>[2x]MFQQLSARLQEAIGRLRGRGRITEEDLKATLREIRRALMDADVNLEVARDFVERVREEALGKQVLESLTPAEVILATVYEALKEALGGEARLPVLKDRNLWFLVGLQGSGKTTTAAKLALYYKGKGRRPLLVAADTQRPAAREQLRLLGEKVGVPVLEVMDGESPESIRRRVEEKARLEARDLILVDTAGRLQIDEPLMGELARLKEVLGPDEVLLVLDAMTGQEALSVARAFDEKVGVTGLVLTKLDGDARGGAA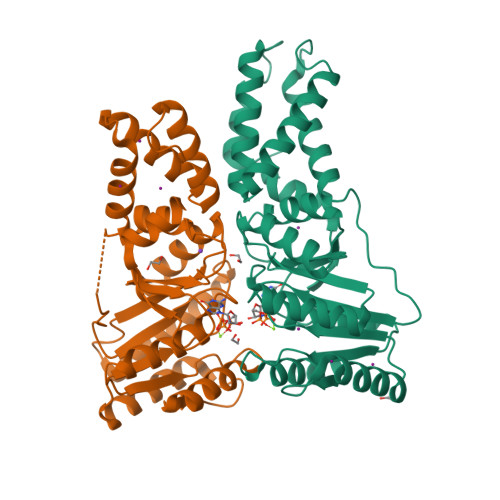LSARHVTGKPIYFAGVSEKPEGLEPFYPERLAGRILGM;>IPWGGNLEEVLEELEMALLAADVGLSATEEILQEVRASGRKDLKEAVKEKLVGMLEPDERRATLRKLGFNPQKPKPVEPKGRVVLVVGVNGVGKTTTIAKLGRYYQNLGKKVMFCAGDTFRAAGGTQLSEWGKRLSIPVIQGPEGTDPAALAYDAVQAMKARGYDLLFVDTAGRLHTKHNLMEELKKVKRAIAKADPEEPKEVWLVLDAVTGQNGLEQAKKFHEAVGLTGVIVTKLDGTAKGGVLIPIVRTLKVPIKFVGVGEGPDDLQPFDPEAFVEALLED[2x]>MARFEEQKLYIGGRYVEASSGATFETINPANGEVLAKVQRASREDVERAVQSAVEGQKVWAAMTAMQRSRILRRAVDILRERNDELAALETLDTGKPLAETRSVDIVTGADVLEYYAGLVPAIEGEQIPLRETSFVYTRREPLGVVAGIGAWNYPVQIALWKSAPALAAGNAMIFKPSEVTPLTALKLAEIYTEAGVPDGVFNVLTGSGREVGQWLTEHPLIEKISFTGGTSTGKKVMASASSSSLKEVTMELGGKSPLIIFPDADLDRAADIAVMANFFSSGQVCTNGTRVFIHRSQQARFEAKVLERVQRIRLGDPQDENTNFGPLVSFPHMESVLGYIESGKAQKARLLCGGERVTDGAFGKGAYVAPTVFTDCRDDMTIVREEIFGPVMSILVYDDEDEAIRRANDTEYGLAAGVVTQDLARAHRAIHRLEAGIC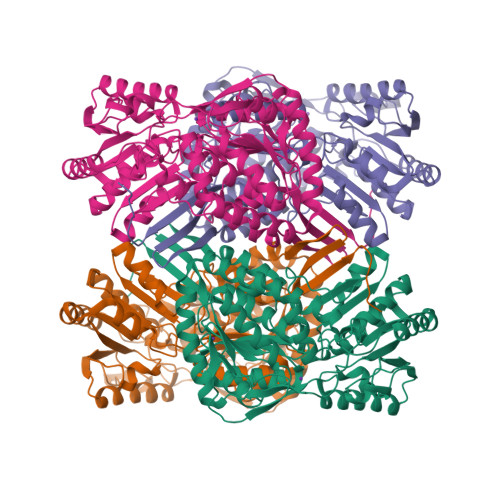WINTWGESPAEMPVGGYKQSGVGRENGLTTLAHYTRIKSVQVELGDYASVF[8x]>MPREIRLPESSVVVRPAPMESATYSQSSRLQAAGLSPAITLFEKAAQTVPLPDAPQPVVIADYGVATGHNSLKPMMAAINALRRRIREDRAIMVAHTDVPDNDFTALFRTLADDPDSYLHHDSASFASAVGRSFYTQILPSNTVSLGWSSWAIQWLSRIPAGAPELTDHVQVAYSKDERARAAYAHQAATDWQDFLAFRGRELCPGGRLVVLTMALDEHGHFGYRPMNDALVAALNDQVRDGLLRPEELRRMAIPVVARAEKDLRAPFAPRGWFEGLTIEQLDVFNAEDRFWAAFQSDGDAESFGAQWAGFARAALFPTLA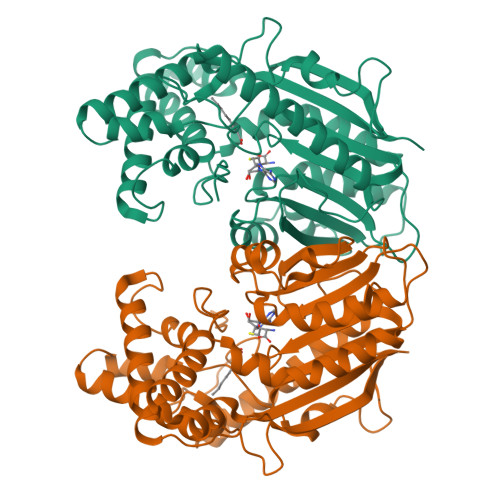AALDCGTGDPRATAFIEQLEASVADRLASQPEPMRIPLASLVLAKRA[2x]> SMAEIKQGIREVILCKDQDGKIGLRLKSIDNGIFVQLVQANSPAS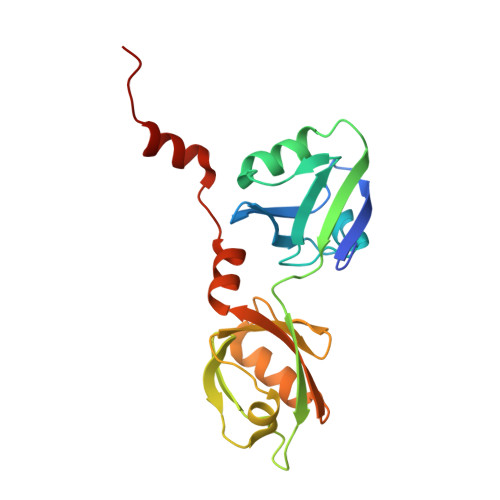LVGLRFGDQVLQINGENCAGWSSDKAHKVLKQAFGEKITMTIRDRPFERTITMHKDSTGHVGFIFKNGKITSIVKDSSAARNGLLTEHNICEINGQNVIGLKDSQIADILSTSGTVVTITIMPAFIFEHIIKRMAPSIMKSLMDHTIPEV> GHMAKAYKQAGVDIEAGYQAVALMKEHVQKTMRPEVLGGIGGFGGLFDLSALGYRQPVLISGTDGVGTKLKLAFLLDRHDTIGIDCVAMCVNDIIVQGAEPLFFLDYIACGKAVPEK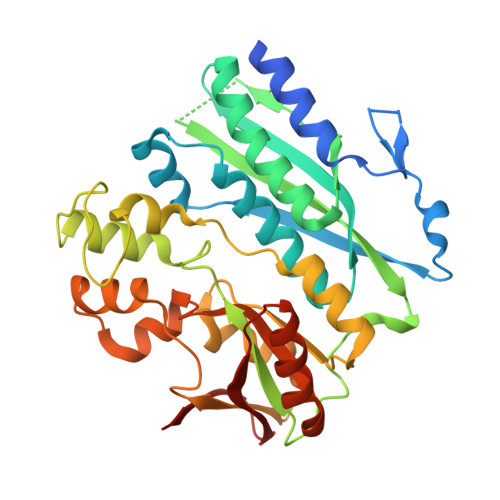IAAIVKGVADGCVEAGCALIGGETAEMPGMYDEDEYDLAGFAVGVAEKERLITGETIQAGDALVGLPSSGLHSNGYSLVRRIVFEQAKLSLDEIYEPLDVPLGEELLKPTRIYAKLLRSVRERFTIKGMAHITGGGLIENIPRMLPPGIGARIQLGSWPILPIFDFLREKGSLEEEEMFSVFNMGIGLVLAVSPETAAPLVEWLSERGEPAYIIGEVAKGAGVSFAGGGRA> XS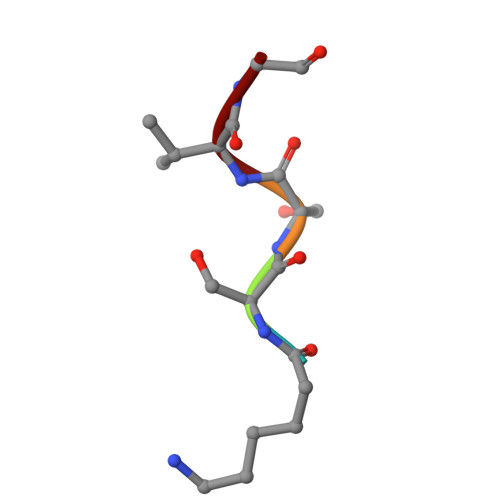SVG> GSHMASFNGVSEAELLTKTLPDILTFNLDIVIIGINPGLMAAYKGHHYPGPGNHFWKCLFMSGLSEVQLNHMDDHTLPGKYGIGFTNMVERTTPGSKDLSSKEFREGGRILVQKLQKYQPRIAVFN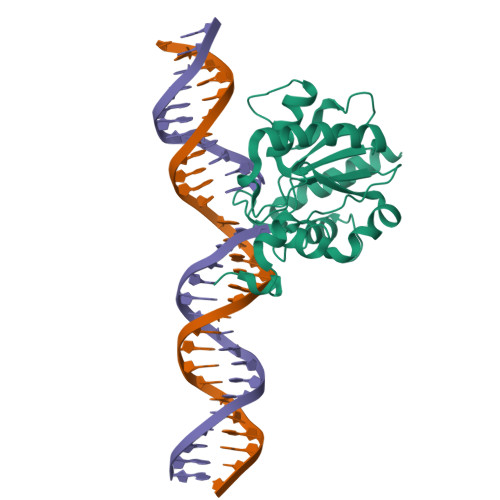GKCIYEIFSKEVFGVKVKNLEFGLQPHKIPDTETLCYVMPSSSARCAQFPRAQDKVHYYIKLKDLRDQLKGIERNMDV> MAHHHHHHVGTMKRKTGFFFDERCFWHSTGLHAVTLPVGGWVQPPAGGGHAESPETKRRMKNLMDVSGLTPQLALRSAAPASLEDLRRIHPDSYLERFKAISDNGGGMLGKEAPLGPGSYEIACLSAGLACAAVEAVLKGELDNAYSLSRPPGHHCLPDQSMGFCFLANIPIAVERAKAQLGLGKVAIIDWDVHHGNGTQHIYLQRDDVLTISLHQDGCFPPGYAGEDDRGVGAGEGYNINIPLLAGAGDDSWRYALETIVIPALARFEPELIIIACGYDANAMDPLARMQLHSDSFRAMTEQVQQAADRLCGGKLVMVHEGGYAESYVPFCGLAVMEALSGIRTEVQDPLLEFIQQQQPRATFAQFQRQAIDRLAQQFGLQ

Classical Zn2+-dependent deac(et)ylases play fundamental regulatory roles in life and are well characterized in eukaryotes regarding their structures, substrates and physiological roles. Structurally, these enzymes are composed of a central eight-stranded parallel β-sheet flanked by α-helices on each site, known as the α/β-arginase/deacetylase fold. All active site residues were conserved, as shown by the multiple sequence alignment and the structural alignment, suggesting a general acid/base catalytic mechanism for the bacterial enzymes as described for the eukaryotic counterparts. These enzymes mediate catalysis using a penta-coordinated catalytic Zn2+ ion coordinated by two aspartates and a histidine (KpHdaH (1b): Asp181, Asp269, His183).

The enzyme KpHdaH (1b) was soaked with SAHA and TSA. We solved the X-ray crystal structures of KpHdaH (1b), RwDmhA (1b), and VcHdaH (5b) in complexes with SAHA to a resolution of 1.95 Å, 1.75 Å, and 1.64 Å, respectively. As described for mammalian Zn2+-dependent HDACs, the hydroxamates coordinated the catalytic Zn2+-ion in a bidentate fashion, the carbonyl oxygen replacing the carbonyl oxygen of the acetamide in the substrate and the hydroxyl group replacing the position of the catalytic water molecule. For all structures, we confirmed the binding of the inhibitors within the substrate binding tunnel with the catalytically important Y of the XGGY-motif forming a hydrogen bond to the carbonyl oxygen of the hydroxamate group. KpHdaH (1b) forms a hydrogen bond with the side chain of Thr24 of the L1-loop with the carbonyl/amide oxygen present in the linker of TSA/SAHA connecting the head group of SAHA and TSA and the hydoxamate warhead. Thr24 contributes to the observed high potency observed for SAHA and TSA to inhibit KpHdaH (1b) activity. This Thr24 is not conserved in bacterial deacylases, exemplifying differences in substrate specificity or inhibition due to differences in structure and sequence of bacterial deacylases. Inspection of the structures of the KpHDAH (1b)•SAHA, KpHDAH (1b)•TSA and RwDmhA (1b)•SAHA showed that the binding site of the inhibitors is created by part of the L1-loop supplied in cis, and by the C-terminal α-helix supplied in trans, i.e. by another monomer of the oligomer. The hydrophobic sequence motif 345-AW-346 in RwDmhA (1b) is substituted by the less hydrophobic sequence motif 356-AQ-357 in VsHdaH (1b) and the hydrophilic sequence motif 346-QQ-347 in KpHdaH (1b).Two proteins, HdeA and HdeB, were discovered as abundant periplasmic proteins in stationary-phase Escherichia coli cells, and genetic studies implicated them in survival of extremely acid pH. HdeA and HdeB have been shown, in vitro, to have acid-activated chaperone functions; that is, by binding to acid-denatured proteins, they prevent these other proteins from irreversible aggregation and precipitation. Like HdeA, HdeB is dimeric at neutral pH but forms monomers at low pH (∼ pH 3.5). We have determined the structure of HdeB and the mechanism of its acid sensing, identifying two critical salt bridges that are broken upon exposure to low pH.

Here, we report the crystal structure of HdeB at pH 4.5 and biophysical characterization of HdeB at both acid and neutral pH. The asymmetric unit of the crystal contains four protein monomers with residues A30 to A102 ordered; six C-terminal residues and the His-tag are disordered. The monomeric structure is composed of two 12-residue helices (α2 and α3), three short (4 or 5 residues) helices (α1, α4, and α5), and interconnecting loops. Analysis with PISA13 reveals that the four monomers in the asymmetric unit are arranged as two identical dimers of HdeB. The dimer is identified as stable by the program PISA13 and the dimer interface buries in total 2400 Å2 of surface area, much of it involving hydrophobic residues. There are six main-chain intersubunit hydrogen bonds (akin to a β-sheet interaction) formed between the loop from each monomer that connects the two long helices. Two tryptophan residues (W55 and W56) and a tyrosine residue (Y64) from each monomer come together to make a cluster of aromatic residues at the C-terminal end of α2. The crystal structure shows an intersubunit salt bridge at the dimer interface of HdeB: E41 from one subunit with K48 from the other and internal salt bridge within each monomer D76–H59. Asp76 makes a polar contact with the indole nitrogen of Trp55 and a salt bridge with His59, which in turn stacks against the indole of W55. The two α2 helices in the HdeA dimer are almost parallel, whereas they are almost perpendicular in the HdeB dimer.

>ANESAKDMTCQEFIDLNPKAMTPVAWWMLHEETVYKGGDTVTLNETDLTQIPKVIEYCKKNPQKNLYTFKNQASNDLPN[4x]> SNAMDGEYHSPYGDDDLYTVQPTERSPRDPKAGEDVILNITTWPIENGQDVWVEWTKNGVAQENVTAAYDYNSGNNTYWKADLGKFEKGDEITYTTKGSTNGGTAYESGPFTFYVTDWEYVQDVTSVVDNGDSITLNMTATAGDFSPKLYLSFEDLDTLRMELSPTGKETGHAGKSGYTVEDTAEKVTVTTEDLSIEIQKSPYRMEVHQADGTLLTSEYTTANSLGWLTDGKNVINQYQNNFMTPSDEAFYGFGERYDTINQRGKDVETYVYNEYQDQAQTERTYLAVPFFVSANKYGMYVNSDFHSQFQMASKVEDKYSFVLDNDGDMTNMLDYYVISGKDQNDIVNNYTDITGKTTLLPKWAFGLWMSANEWDRESDVSSALSNAKANDIPATGFVLEQWSDEETYYIWNNATYTAKKNGEAFSYDDFTFNGKWTDPKGMVDSVHDAGMNIVLWQVPVLKDDGTVYEQRDNDEEYMISQGYSADDGTGAPYRVPASQWFGNGILLDFTNKDAVDWWTSQREYLLTEVGIDGFKTNGGEMVWGRDTTFSNGEKGQEMRNRYPTDYVSSYFDFAKSINPEAVSFSRSGTSGAQKSGIYWSGDQTSTFDSFQASLKAGLSASTSGVSYW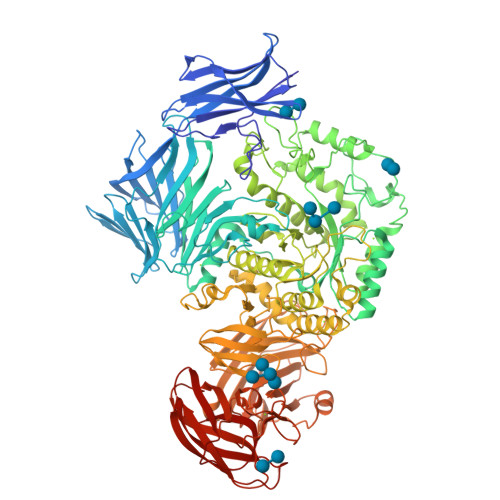AWDMAGFTGDYPTAELYKRATAMAAFAPIMQFHSEKSDPSPSEERSPWNAVARTGDETILPTFQKYLYTRMNLLPYIYTAAKDTADNGKSMMRQMAMDYPEDVNARDLDEQYMFGDDLLVAPIVQEGQTEKEVYLPEGEWVDIWNGGVHPGGETISYYADVDTLPVFAKAGAIIPMNMTDGYQLGQNVGNDLKSYDNLTFRVYPSGDSEYSFYDDVNGGEMRDISVSEDFANEKVSVDLPAMADETTMQVFSTEPTSVTIDGADVAKADTLDAFNEATTGYYYDTVQNLTYVKAAAKDAKQAIVLNGVNHAPYEAEFGHLTNVTTASDHAGYTGTGFVAGFDAEKEAVEFDIDAVDGASDYTMEVRYSAGVEDATRTVYINGKKQQITLPKTANWDTWNTVEVPVTLQAGNNQVVFDFEADDTAGINFDHVVIKK>MEKKHIYLFSSA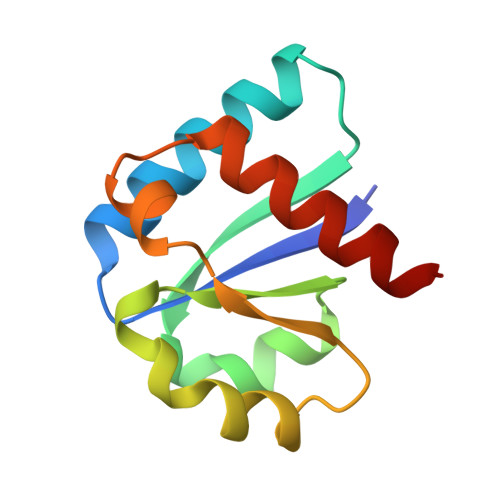GMSTSLLVSKMRAQAEKYEVPVIIEAFPETLAGEKGQNADVVLLGPQIAYMLPEIQRLLPNKPVEVIDSLLYGKVDGLGVLKAAVAAIKKAAAN[2x]> M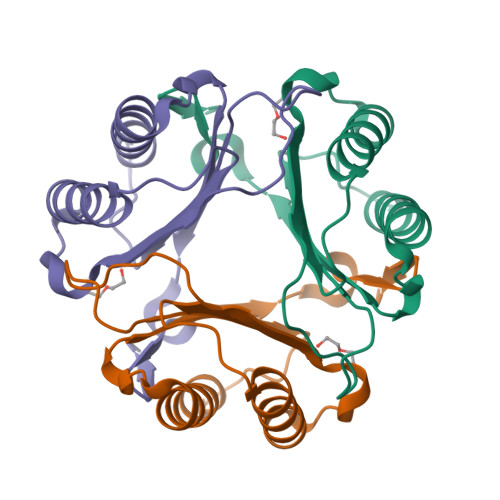PLINIQASVPAVADANSLLQELSSKLAELLGKPEKYVMTSLQCGVPMTFSGNTEPTCYVEVKSIGALDGSRTQEVSELVCGHIEQNLGIPADRIYIGFEDVPARLWGWNGSTFG> MGSSHHHHHHSSGLVPRGSHMASDEGLKNEIKNNDITKDISIYPTPKDMTVGNSEFTLEDSVNIVGGDLADTYAFELLKNMLTEFGIKINESEIEGATTIYIGESDDNIEEMENTLEEMNVDTSSISKDEGYVLVTDENTEGNKIVIRGNDETGTFYGVKSLKQLIKKEDNKVILDEVVIKDEPSFKMRAVVEGFYGTPWSQEERLDQIKMYGEYKMNAYIYAPKSDPYHREKWREPYPASELDRMKELIKTANENKVDFVFAISPGLDIKFEGEEGEADFKALINKAETLYDMGVRSFAILWDDIENRSGVQQAEVLNRFNKEFIKNKEGVKPLITVPVEYWGSSMFNGEEVKTYTKEFAETLDKDIEVMWTGNDVIPPNGVSLEDAKKVSNVYNRKMMLWWNYPV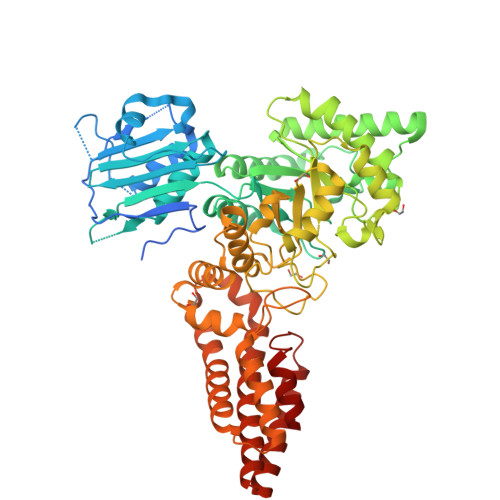NDYKEDKMALGPIYDLDRNLDEEVSGFIVNPMRFSDASKISTLTGADYGWNSVSYEAEKSWDKAIEIIAGEMKEEFKIFANHSTRLDTGRPDSPEIKNTIDSLWEKWEAGSDISLELSNLQNEFSKMVQVPNKLRSNLENKALLNQLDSHLSKFEIYGNAGLKSIEILQDIVNKDMSEFWSDNFEGIKLLRNLDGIKATIANNVVDPFIRKVHE4-HYDROXY-7-METHOXY-3-(1-PHENYL-PROPYL)-CHROMEN-2-ONE | C19 H18 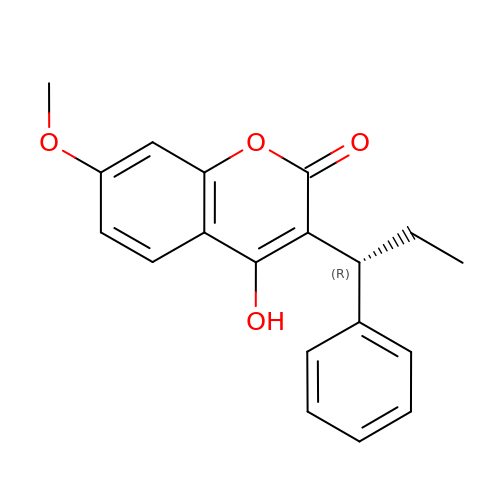O4 | CCPGCKQLIHGSCJ-AWEZNQCLSA-N>CGCG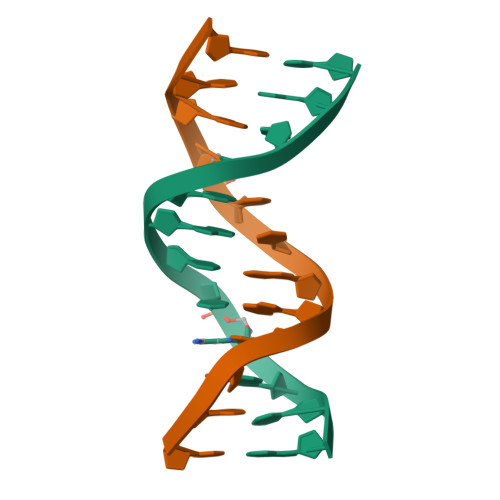AATTAGCG[2x]> ANIVGGIEYSINNASLCSVGFSVTRGATKGFVTAGHCGTVNATARIGGAVVGTFAARVFPGNDRAWVSLTSAQTLLPRVANGSSFVTVRGSTEAAVGAAVCRSGRTTGYQCGTITAKNVTANYAEGAVRGLTQGNACAGRGDSGGSWITSAGQAQGVMSGLNVQSNGNNCGIPASQRSSLFERLQPILSQYGLSLVTG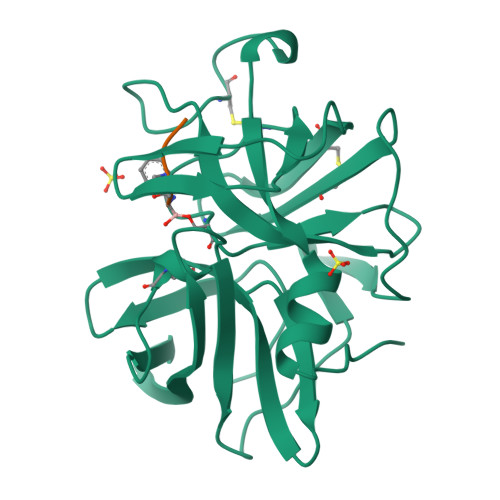;> XAAPF>[2x]GSEKLGKLQYSLDYDFQNNQLLVGIIQAAELPALDMGGTSDPYVKVFLLPDKKKKFETKVHRKTLNPVFNEQFTFKVPYSELAGKTLVM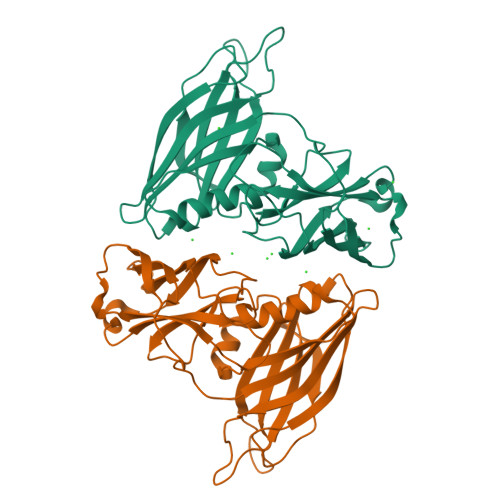AVYDFDRFSKHDIIGEFKVPMNTVDFGHVTEEWRDLQSAEKEEQEKLGDICFSLRYVPTAGKLTVVILEAKNLKKMDVGGLSDPYVKIHLMQNGKRLKKKKTTIKKNTLNPYYNESFSFEVPFEQIQKVQVVVTVLDYDKIGKNDAIGKVFVGYNSTGAELRHWSDMLANPRRPIAQWHTLQVEEEVDAMLAVKK Acetyl xylan esterases (EC 3.1.1.72; AXEs) catalyze the specific hydrolysis of the ester linkages between the xylose units and acetic acid, facilitating the access of main chain depolymerizing enzymes. We identified a novel acetyl xylan esterase (PbAcE) belonging to the CE7 family from this strain. Here, we present the first crystal structure of a cold-adapted acetyl xylan esterase from the psychrophilic soil microbe Paenibacillus sp. R4. However, PbAcE, which is derived from a psychrophilic microorganism, showed the highest activity at 4°C, suggesting that its structural and biochemical properties are optimized to low temperatures.

The crystal structure of PbAcE belongs to the C2 space group and contains six molecules in the asymmetric unit, forming a donut-shaped hexamer. The central tunnel of the donut-shaped hexamer has a diameter of about 18.5 Å. Each monomer of PbAcE is composed of 11 α-helices and 9 β-strands. The conserved catalytic triad residues of Ser185, Asp274, and His303 are located inside the hexamer tunnel, with a neighboring putative substrate binding site. This hydrophobic putative substrate binding site is composed of β4, β6, and β7 strands and α3 and α11 helices. The β-interface has also been identified at the dimer interfaces of PbAcE. In the PbAcE structure, the L144 residue forms a hydrophobic interaction with Y133, stabilizing the β-interface loop structure. PbAcE has a relatively more open and larger cleft in comparison with those of BsAcE and TmAcE. The B-factor distribution analysis of the PbAcE structure showed that the values of the β4–α3 (residues 93–101) and β5–α4 (residues 119–152) loop regions were lower than the average for the whole PbAcE structure. Notably, the PbAcE β4–α3 and β5–α4 loop structures are one and six residues shorter than those of TmAcE, respectively. These shortened gatekeeper loops may expand the substrate binding site area and create a more open active site conformation.

>[6x]MPNVDMPLSQLQDYKPELTNETDFDLFWDNAKALSNQKPLHAQVNLVQDYPLKSISIYDVVYDGADGTPIHGWYVTPKGEHQPGSLPVLVKYHGYSGNRGYPNELLQWASMGMAALAIDVRGQGGVTPDRAEYPQGGIPGWMTLGILDPASYYYKQVYLDCIRALDFVCSREEVDASRIAVYGGSQGGGLALAAAGLDSRPKLALPVFPFLCHFRRSVEIHASGPYVEIKNWFRRYDPEHRQEEQVYRTLSYFDGMNMASRIKARTLMAITLQDITCPPSTCFAAYNHLAGPKEVRLYHDYGHEGLPFHEEAMMRFIEAYL>[2x]GSHMEPP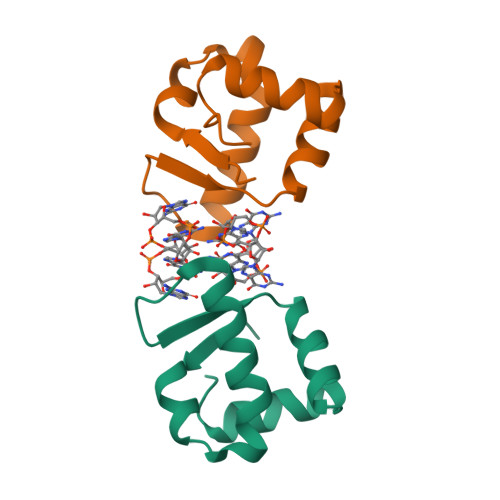PKLVLDLERLATVPAEKAGPLQRYAATIQSQRGDYNGKVLSIRQDDLRTLAVIYDQSPSVLTEQLISWGVLDADARRAVASHDEL4-METHYL-2-OXO-2H-CHROMEN-7-YL 5-(ACETYLAMINO)-3,5-DIDEOXY-L-ERYTHRO-NON-2-ULOPYRANOSIDONIC ACID | C21 H25 N O11 | 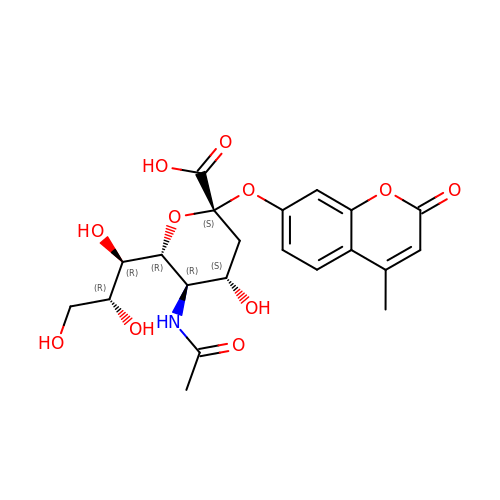KKDWIUJBUSOPGC-GKHMPSLRSA-N>[2x]MELCGLGLPRPPMLLALLLATLLAAMLALLTQVALVVQVAEAARAPSVSAKPGPALWPLPLSVKMTPNLLHLAPENFYISHSPNSTAG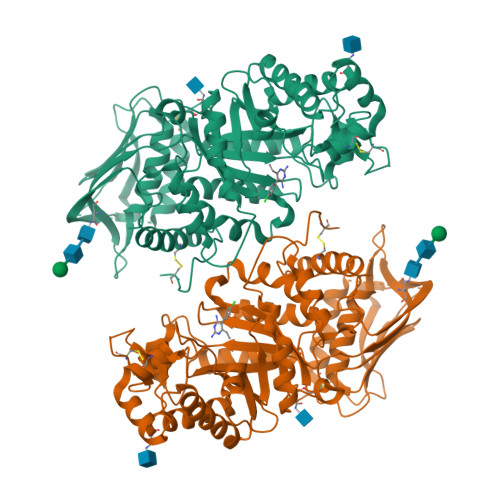PSCTLLEEAFRRYHGYIFGFYKWHHEPAEFQAKTQVQQLLVSITLQSECDAFPNISSDESYTLLVKEPVAVLKANRVWGALRGLETFSQLVYQDSYGTFTINESTIIDSPRFSHRGILIDTSRHYLPVKIILKTLDAMAFNKFNVLHWHIVDDQSFPYQSITFPELSNKGSYSLSHVYTPNDVRMVIEYARLRGIRVLPEFDTPGHTLSWGKGQKDLLTPCYSRQNKLDSFGPINPTLNTTYSFLTTFFKEISEVFPDQFIHLGGDEVEFKCWESNPKIQDFMRQKGFGTDFKKLESFYIQKVLDIIATINKGSIVWQEVFDDKAKLAPGTIVEVWKDSAYPEELSRVTASGFPVILSAPWYLDLISYGQDWRKYYKVEPLDFGGTQKQKQLFIGGEACLWGEYVDATNLTPRLWPRASAVGERLWSSKDVRDMDDAYDRLTRHRCRMVERGIAAQPLYAGYCNHENM MRV is a prototypical member of the Reoviridae family of segmented double-stranded RNA (dsRNA) viruses, which is further divided into two subfamilies based on the presence or absence of turrets on the inner capsids: turreted (Spinareovirinae, including MRV) and nonturreted (Sedoreovirinae, including bluetongue virus (BTV) and the life-threatening rotavirus). MRV capsids are composed of two concentric protein layers, encapsulating 10 dsRNA segments. The outer layer of MRV consists of the protection protein σ3, membrane penetration protein μ1, and spike protein σ1. The inner layer consists of proteins λ1, σ2, and turret protein λ223.

Meanwhile, the outer shell particle, consisting of the outer layer proteins μ1, σ3, and λ2, appears to be a byproduct of MRV assembly. The outer shell particle appears to be a byproduct of assembly, as it lacks any inner layer proteins or RNA genome. This notion is supported by our single-particle analyses of viral isolates (described below), which show a much higher percentage of outer shell particles in the late infection stage as compared to the early infection stage. Analysis of total particle abundance from the two-time points shows that the proportion of single-layered particles decreases between the 6 and 48 h post-infection points (4.1% vs 1.3%), while the proportion of outer shell particles increases dramatically during that time (0.5% vs 22.5%).

>MGNASSIVQTINVTGDGNVFKPSAETSSTAVPSLSLSPGMLNPGGVPWIAVGDETSVTSPGALRRMTSKDIPETAIINTDNSSGAVPSESALVPYIDEPLVVVTEHAITNFTKAEMALEFNREFLDKMRVLSVSPKYSDLLTYVDCYVGVSARQALNNFQKQVPVITPTRQTMYVDSIQAALKALEKWEIDLRVAQTLLPTNVPIGEVSCPMQSVVKLLDDQLPDDSLIRRYPKEAAVALAKRNGGIQWMDVSEGTVMNEAVNAVAASALAPSASAPPLEEKSKLTEQAMDLVTAAEPEIIASLAPVPAPVFAIPPKPADYNVRTLRIDEATWLRMIPKSMNTPFQIQVTDNTGTNWHLNLRGGTRVVNLDQIAPMRFVLDLGGKSYKETSWDPNGKKVGFIVFQSKIPFELWTAASQIGQATVVNYVQLYAEDSSFTAQSIIATTSLAYNYEPEQLNKTDPEMNYYLLATFIDSAAITPTNMTQPDVWDALLTMSPLSAGEVTVKGAVVSEVVPADLIGSYTPESLNASLPNDAARCMIDRASKIAEAIKIDDDAGPDEYSPNSVPIQGQLAISQLETGYGVRIFNPKGILSKIASRAMQAFIGDPSTIITQAAPVLSDKNNWIALAQGVKTSLRTKSLSAGVKTAVSKLSSSESIQNWTQGFLDKVSAHFPAPKPDCPTSGDSGESSNRRVKRDSYAGVVKRGYTR[6x];>[3x]MEVCLPNGHQVVDLINNAFEGRVSIYSAQEGWDKTISAQPDMMVCGGAVVCMHCLGVVGSLQRKLKHLPHHRCNQQIRHQDYVDVQFADRVTAHWKRGMLSFVAQMHEMMNDVSPDDLDRVRTEGGSLVELNWLQVDPNSMFRSIHSSWTDPLQVVDDLDTKLDQYWTALNLMIDSSDLIPNFMMRDPSHAFNGVKLGGDARQTQFSRTFDSRSSLEWGVMVYDYSELEHDPSKGRAYRKELVTPARDFGHFGLSHYSRATTPILGKMPAVFSGMLTGNCKMYPFIKGTAKLKTVRKLVEAVNHAWGVEKIRYALGPGGMTGWYNRTMQQAPIVLTPAALTMFPDTIKFGDLNYPVMIGDPMILG;> MANVWGVRLADSLSSPTIETRTRQYTLHDLCSDLDANPGREPWKPLRNQRTNNIVAVQLFRPLQGLVLDTQLYGFPGAFDDWERFMREKLRVLKYEVLRIYPISNYSNEHVNVFVANALVGAFLSNQAFYDLLPLLIINDTMIGDLLGTGASLSQFFQSHGDVLEVAAGRKYLQMENYSNDDDDPPLFAKDLSDYAKAFYSDTYEVLDRFFWTHDSSAGVLVHYDKPTNGHHYLLGTLTQMVSAPPYIINATDAMLLESCLEQFSANVRARPAQPVTRLDQCYHLRWGAQYVGEDSLTYRLGVLSLLATNGYQLARPIPRQLTNRWLSSFVSQIMSDGVNETPLWPQERYVQIAYDSPSVVDGATQYGYVRKNQLRLGMRISALQSLSDTPSPVQWLPQYTIDQAAMDEGDLMVSRLTQLPLRPDYGNIWVGDALSYYVDYNRSHRVVLSSELPQLPDTYFDGDEQYGRSLFSLARKIGDRSLVKDTAVLKHAYQAIDPNTGKEYLRSRQSVAYFGASAGHSGADQPLVIEPWIQGKISGVPPPSSVRQFGYDVARGAIVDLARPFPSGDYQFVYSDVDQVVDGHDDLSISSGLVESLLSSCMHATAPGGSFVVKINFPTRPVWHYIEQKILPNITSYMLIKPFVTNNVELFFVAFGVHQHSSLTWTSGVYFFLVDHFYRYETLSTISRQLPSFGYVDDGSSVTGIETISIENPGFSNMTQAARIGISGLCANVGNARKSIAIYESHGARVLTITSRRSPASARRKSRLRYLPLIDPRSLEVQARTILPADPVLFENVSGASPHVCLTMMYNFEVSSAVYDGDVVLDLGTGPEAKILELIPATSPVTCVDIRPTAQPSGCWNVRTTFLELDYLSDGWITGVRGDIVTCMLSLGAAAAGKSMTFDAAFQQLIKVLSKSTANVVLVQVNCPTDVVRSIKGYLEIDSTNKRYRFPKFGRDEPYSDMDALEKICRTAWPNCSITWVPLSYDLRWTRLALLESTTLSSASIRIAELMYKYMPIMRIDIHGLPMEKRGNFIVGQNCSLVIPGFNAQDVFNCYFNSALAFSTEDVNAAMIPQVSAQFDATKGEWTLDMVFSDAGIYTMQALVGSNANPVSLGSFVVDSPDVDITDAWPAQLDFTIAGTDVDITVNPYYRLMTFVRIDGQWQIANPDKFQFFSSASGTLVMNVKLDIADKYLLYYIRDVQSRDVGFYIQHPLQLLNTITLPTNEDLFLSAPDMREWAVKESGNTICILNSQGFVLPQDWDVLTDTISWSPSIPTYIVPPGDYTLTPL>[3x]MIQGVIQKIAGPAVIAKGMLGARMYDICKVGEEGLVGEIIRLDGDTAFVQVYEDTSGLKVGEPVVSTGLPLAVELGPGMLNGIYDGIQRPLERIREKTGIYITRGVVVHALDREKKWAWTPMVKPGDEVRGGMVLGTVPEFGFTHKILVPPDVRGRVKEVKPAGEYTVEEPVVVLEDGTELKMYHTWPVRRARPVQRKLDPNTPFLTGMRILDVLFPVAMGGTAAIPGPFGSGKTVTQQSLAKWSNADVVVYVGCGERGNEMTDVLVEFPELTDPKTGGPLMHRTVLIANTSNMPVAAREASIYVGVTIAEYFRDQGFSVALMADSTSRWAEALREISSRLEEMPAEEGYPPYLAARLAAFYERAGKVITLGGEEGAVTIVGAVSPPGGDMSEPVTQSTLRIVGAFWRLDASLAFRRHFPAINWNGSYSLFTSALDPWYRENVAEDYPELRDAISELLQREAGLQEIVQLVGPDALQDAERLVIEVGRIIREDFLQQNAYHEVDAYCSMKKAYGIMKMILAFYKEAEAAIKRGVSIDEILQLPVLERIGRARYVSEEEFPAYFEEAMKEIQGAFKAL;>EYTGITYISGPLLFVENAKDLAYGAIVDIKDGTGRVRGGQVIEVSEEYAVIQVFEETTGLDLATTSVSLVEDVARLGVSKEMLGRRFNGIGKPIDGLPPITPEKRLPITGLPLNPVARRKPEQFIQTGISTIDVMNTLVRGQKLPIFSGSGLPANEIAAQIARQATVRPDLSGEGEKEEPFAVVFAAMGITQRELSYFIQEFERTGALSRSVLFLNKADDPTIERILTPRMALTVAEYLAFEHDYHVLVILTDMTNYCEALREIGAAREEIPGRRGYPGYMYTDLATIYERAGVVEGKKGSVTQIPILSMPDDDRTHPIPDLTGYITEGQIQLSRELHRKGIYPPIDPLPSLSRLMNNGVGKGKTREDHKQVSDQLYSAYANGVDIRKLVAIIGEDALTENDRRYLQFADAFERFFINQGQQNRSIEESLQIAWALLSMLPQGELKRISKDHIGKYY[3x];>[2x]KLEAILSQEVEAEIQALLQEAEAKAEAVKREAEEKAKALLQARERALEAQYRAALRRAESAGELLVATARTQARGEVLEEVRRRVREALEALPQKPEWPEVVRKLALEALEALPGAKALVANPEDLPHLEAMARERGVELQAEPALRLGVRAVGAEGKTQVENSLLARMDRAWDAMSSKVAQALWG;>GMGGLGLIKSLAEKEKQLLERLEAAKKEAEERVKRAEAEAKALLEEAEAKAKALEAQYRERERAETEALLARYRERAEAEAKAVREKAMARLDEAVALVLKEVLP[2x];> SQVSPTRMNLLQRRGQLRLAQKGVDLLKKKRDALVAEFFGLVREAMEARKALDQAAKEAYAALLLAQAFDGPEVVAGAALGVPPLEGVEAEVENVWGSKVPRLKATFPDGALLSPVGTPAYTLEASRAFRRYAEALIRVANTETRLKKIGEEIKKTTRRVNALEQVVIPGIRAQIRFIQQVLEQREREDTFRLKRIKGKIEAREAEEEGG;> MAVIADPETAQGFRLAGLEGYGASSAEEAQSLLETLVERGGYALVAVDEALLPDPERAVERLMRGRDLPVLLPIAGLK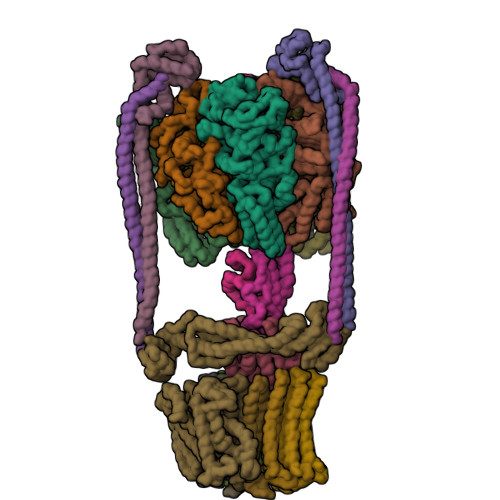EAFQGHDVEGYMRELVRKTIGF;> MADDFAYLNARVRVRRGTLLKESFFQEALDLSFADFLRLLSETVYGGELAGQGLPDVDRAVLRTQAKLVGDLPRLVTGEAREAVRLLLLRNDLHNLQALLRAKATGRPFEEVLLLPGTLREEVWRQAYEAQDPAGMAQVLAVPGHPLARALRAVLRETQDLARVEALLAKRFFEDVAKAAKGLDQPALRDYLALEVDAENLRTAFKLQGSGLAPDAFFLKGGRFVDRVRFARLMEGDYAVLDELSGTPFSGLSGVRDLKALERGLRCVLLKEAKKGVQDPLGVGLVLAYVKEREWEAVRLRLLARRAYFGLPRAQVEEEVVCP;> MIAPMEKLVLAGPKGRAKELLQSLQQAGVVHLETLRPEALSAYQLSPEERAELRRWEAVSAGAEHTLSLLGLEAEPARPFPEGLEAAEKALSPIQAHAEGLTRQKQELEEELALAQAYLEPLERLAALAHGLDKSPFLRVIPFLLTEKELPLVEEALRKALEDRYLLAHEAYAGGVPALVVVHRKEVDQAKAALSRAGVAELRLPGALGELPLSEAARRLKERAEAAPRELSEVRQHLAKLARESASTLQSLWTRAQDEVARLKALEELASGRFGFALLGYVPVKAKPKVEEALARHKENVVYAFEPVDEHHEADRIPVVLDNPPWVKPFELLVSFLNTPKYGTFDPTPVVPIFFPFWFGMIVGDIGYALLFYLVGRWLSGYVKRNEPLVIDLFALKLKPPVLAKLVYILNWMVFWTVVWGLIYGEFFGTFLEHLGVFGTPEHPGLIPILIHRIDTAKTANLLILLSVAFGVVMVFAGLILRAYLGLKHRHMAHFWEGVGYLGGLLGILALAASYLGNLQAGWLSALMYLGFGVFLLSVVMSSIWLMIPEIFTQAGHILSHIRIYAVGAAGGILAGLLTDVGFAMAERLGLIGVLLGIVVAGVLHLLILLLTTLGHMLQPIRLIWVEFFTKFGFYEENGRPYRPFKSVRETQ;>[12x]MKKLLVTVLLAVFGALAFAAEEAAASGGLDRGLIAVGMGLAVGLAALGTGVAQARIGAAGVGAIAEDRSNFGTALIFLLLPETLVIFGLLIAFILNGRL Here we describe extendable linear, curved and angled protein building blocks, as well as inter-block interactions, that conform to specified geometric standards; assemblies designed using these blocks inherit their extendability and regular interaction surfaces, enabling them to be expanded or contracted by varying the number of modules, and reinforced with secondary struts. We construct twistless helix repeat (THR) protein blocks from identical straight α-helices (typically 2–4 helices in each unit); the length of the blocks can be varied simply by varying the number of repeat units. Restricting helical geometry to ideal straight helices with zero helical twist in principle considerably limits what types of structure could be built, but this is more than compensated by the great simplification of downstream material design, as illustrated below. Using X-ray crystallography and electron microscopy, we validate nanomaterial designs ranging from simple polygonal and circular oligomers that can be concentrically nested, up to large polyhedral nanocages and unbounded straight ‘train track’ assemblies with reconfigurable sizes and geometries that can be readily blueprinted.

Expandability over four different sizes was achieved with cage_O43_129 (+0, +4, +8 and +12 helices). The internal structure of the oligomers is clearly resolved in cryo-EM reconstructions for the first three sizes and in ns-EM reconstruction of the largest size; the distance between the centre of mass of the tetramer component to the centre of mass of the trimer component across the different sizes is 7.9, 9.4, 11.3 and 11.7 nm respectively. Views down each of the three symmetry axes (twofold, threefold and fourfold) are clear for each size (except for the threefold view in the largest size) with slight rotational deviations of the fourfold cyclic component compared to the design model, whereas the rotation of the threefold cyclic component holding the THR remains unperturbed as designed.

>[24x]MGCDAIQAAAALGEAGISSNEILELLAAAAELGLDPDAIQAAAQLGEAGISSEEIKELLRAAHELGLDPDAIAAAADLGQAGVSPVEILALLIAASVLGLDPDAIQAAAALGEAGISAEEIIELLTAARDLGLDPDAIQAAAQLGEAGISSEEIKELLRAAHELGLDPDCIAAAADLGQAGISSSEITALLLAAAAIELAKRADDKDVREIVRDALELASRSTNDEVIRLALEAAVLAARSTDSDVLEIVKDALELAKQSTNEEVIKLALKAAVLAAKSTDEEVLEEVKEALRRAKESTDEEEIKEELRKAVEEAEGGSWLEHHHHHH;>[24x]MGDDLLLKLLELLVEQARVSAEFARRQGDEKMLEEVARKAEEVARKAEEIARKARKEGNLELALKALEILVRAAHVLAEIARERGNEELQKKAHKLAKEALRQVIEIAIRAIQEGNLELAIIALHISVRIAEVLLETRPDDREEIREQQAIFELLIAALEAAIRLEKLKEEGAPPEQIERVAEHGLERLKEIAKEISKEVDSPESKRIAYKIVAAAAEFLLKILAEGGATPEQLERVTEHALEVLKEVAKELADSPESVREAVRLISKLTQEGLKQLKEIGAPPEQIERVAEHGLEVLKEIAKYGSKLTDSPELKRELYRIISETAKELLKILAEGGATPEQLERVTKHALEVLKEVAKELADSPESGLAALAAIASLAKLGLEQLKEIGAPPEQQRRVTKAGIEAVREIYRYGRKLY(3~{S},7~{R},10~{R},13~{S})-4-[[(3~{R},7~{S},10~{S},13~{R})-4-[(2~{S})-2-acetamido-3-(2-chlorophenyl)propanoyl]-2-oxidanylidene-1,4-diazatricyclo[8.3.0.0^{3,7}]tridec-8-en-13-yl]carbonyl]-2-oxidanylidene-1,4-diazatricyclo[8.3.0.0^{3,7}]tridec-8-ene-13-carboxylic 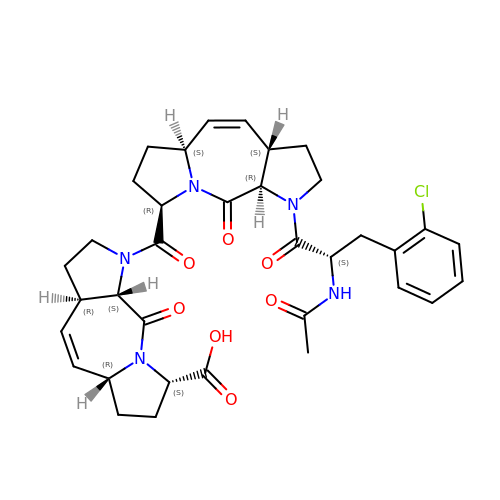acid | C35 H40 Cl N5 O7 | VTQUUKLGUPHTFW-IDZQPSAXSA-N>[4x]MDAKKVAKKAAIQAARRITELAQVLVELLKEALKLDLTQEMRKKLIERYAAAIIRAIGDINNAIYQAKQEAEKLKKAGLVDSDQLDALLRALDELQKVASKAANQLGRLFEEALKRLDKDNGGEEEKDRTAKWFEFEARAIEIALRLAAIGDVFDLEKEWRKLKSRGKL;>[4x]MDE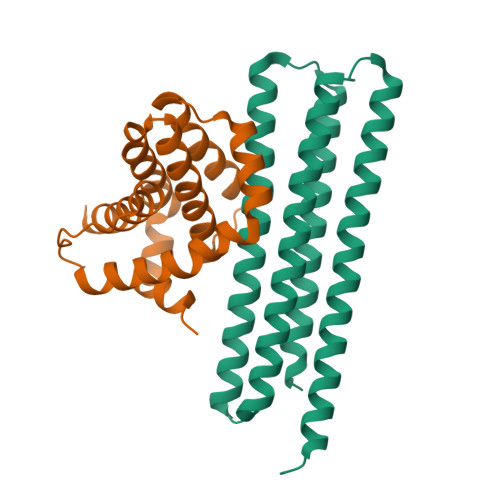LYRQSLEIISRYLREQATGAKDTKPMGRSGATSRKALETLRRVGDGVQRNHETAFQGMLRKLDIKNEDDVKSLSRVMIHVFSDGVTNWGRIVTLISFGAFVAKHLKTINQESCIEPLAESITDVLVRTKRDWLVKQRGWDGFVEFFHVSRGKL>MGSSHHHHHHSSGLVPRGSHMASGLYPSYNTSPAAPDSTGMQSTAVQLAGKIRLG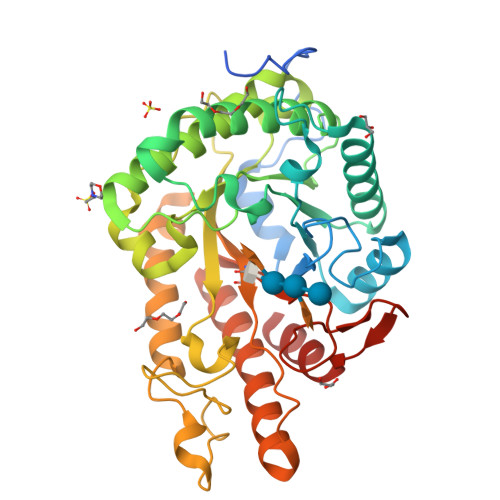WNIGNTMEAIGGETAWGNPMVSNELLKLVKDSGFDAVRIPVAWDQYANQESAEISAAWLNRVKQVVQMAIDNELYVLINIHWDGGWLENNITPAKKDENNAKQKAFWEQIATHLRDFDEHLLFAGTNAPNAENAEQMDVLNSYLQTFVDAVRSTGGKNAYRVLVLQGPVTDIEKTNELWTHMPADTATDRLMAEVHFYTPYNFALMRQDESWGKQFYYWGEGFLSTTDTERNPTWGEEATIDQLFDLMKTKFVDQGIPVVLGEFSAMRRTNLTGDALTLHLAGRAYYHKYVTQQALARGLLPFYWDNGGNDNFSSGIFNRQQNTVFDQQVLDALLEGAGAQ[2x]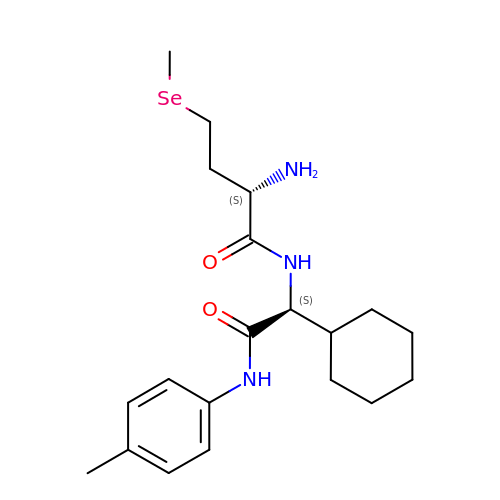(2S)-2-amino-N-{(1S)-1-cyclohexyl-2-[(4-methylphenyl)amino]-2-oxoethyl}-4-(methylselanyl)butanamide | C20 H31 N3 O2 Se | VAUYIWWHFJNKTF-ROUUACIJSA-N ethyl 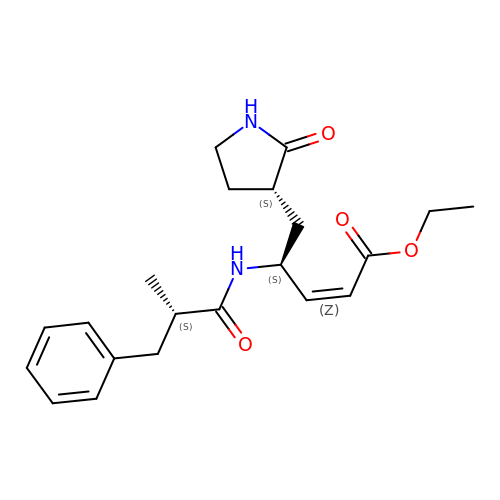(2Z,4S)-4-{[(2S)-2-methyl-3-phenylpropanoyl]amino}-5-[(3S)-2-oxopyrrolidin-3-yl]pent-2-enoate | C21 H28 N2 O4 | XDPDGHIMOBFVDD-RYQLBKOJSA-N>[2x]AQSVPYGISQIKAPALHSQGYTGSNVKVAVIDSGIDSSHPDLNVRGGASFVPSETNPYQDGSSHGTHVAGTIAALNNSIGVLGVAPSASLYAVKVLDSTGSGQYSWIINGIEWAISNNMDVINMSLGGPTGSTALKTVVDKAVSSGIVVAAAAGNEGSSGSTSTVGYPAKYPSTIAVGAVNSSNQRASFSSVGSELDVMAPGVSIQSTLPGGTYGAY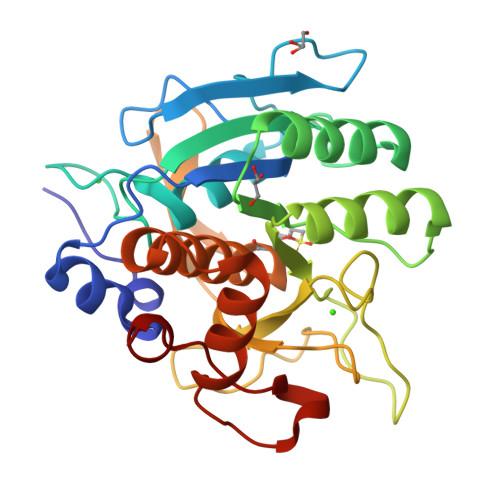NGTSMATPHVAGAAALILSKHPTWTNAQVRDRLESTATYLGNSFYYGKGLINVQAAAQ> GPHMSPDKKWLGTPIEEMRRMPRCGIRLPLLRPSANHTVTIRVDLLRAGEVPKPFPTHYKDLWDNKHVKMPCSEQNLYPVEDENGERTAGSRWELIQTALLNKFTRPQNLKDAILKYNVAYSKKWDFTALIDFWDKVLEEAEAQHLYQSILPDMVKIALCLPNICTQPIPLLAAAMNHSITMSQEQIASLLANAFFCTFPRRNAKMKSEYSSYPDINFNRLFEGRSS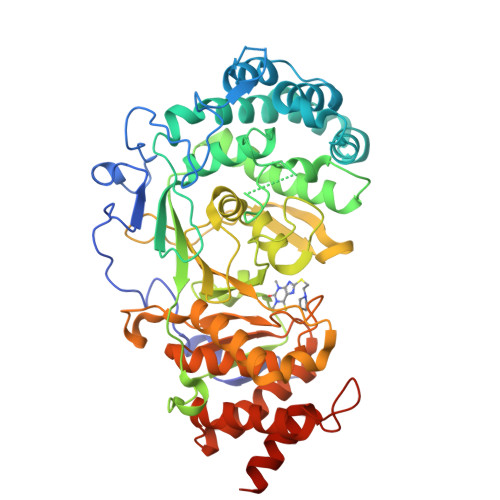RKPEKLKTLFCYFRRVTAAAPTGLVTFTRQSLEDFPEWERCEKPLTRLHVTYEGTIEENGQGMLQVDFANRFVGGGVTSAGLVQEEIRFLINPELIISRLFTEVLDHNECLIITGTEQYSEYTGYAETYRWSRSHEDGSERDDWQRRCTEIVAIDALHFRRYLDQFVPEKMRRELNKAYCGFLRPGVSSENLSAVATGNWGCGAFGGDARLKALIQILAAAAAERDVVYFTFGDSELMRDIYSMHIFLTERKLTVGDVYKLLLRYYNEECRNCSTPGPDIKLYPFIYHAVESCAETADHSGQRTGT> MQIITAEDYRLYGGLKRPELESGVEMMITAANALITSLLGMD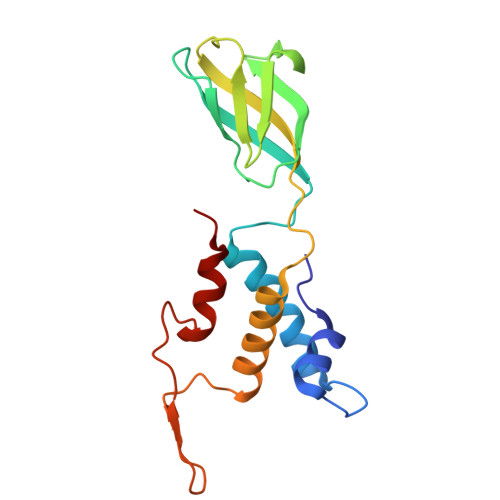DADAVDQLINTKPTRKKYFLSSPSATSVTKMTINDKEIDPEQYKLYSDGVILLKFSPPEGYMDVEYTQGGFNPIPEDLKLAACMLVDHWHKQDYRQAKTIGGETVTFNNTKSGIPEHIRTIIEVYRRV2-AMINO-5-(2,3-DIHYDROTHIENO[3,4-B][1,4]DIOXIN-5-YL)-N-[2-(DIMETHYLAMINO)ETHYL]PYRIDINE-3-CARBOXAMIDE | C16 H20 N4 O3 S | 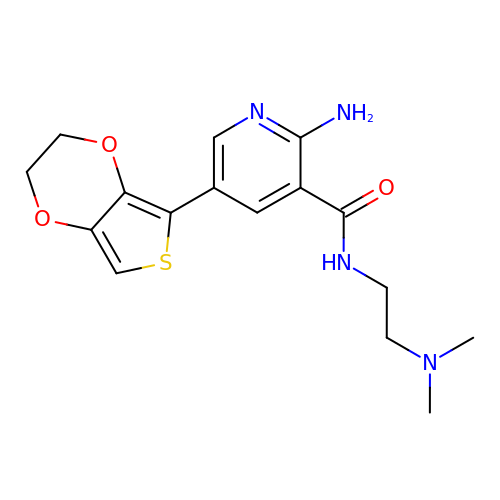XGNFTBBPLXKQQH-UHFFFAOYSA-N By contrast, in vertebrates the clustered protocadherins (Pcdhs) provide analogous cell-surface diversity, but in this case generated through stochastic alternative promoter choice. Biophysical measurements with domain-deleted proteins showed that Pcdhs also interact in cis, through a membrane-proximal dimer interface involving extracellular cadherin domain 6 (EC6) and potentially EC5. The specificity-determining cell-cell recognition interface of Pcdhs involves domains EC1–4, as shown experimentally through mutagenesis analysis and suggested by mutation correlation analysis.

Crystallization screening of these dimeric γ-Pcdh fragments yielded crystals of γA1EC1–4, γA8EC1–4, γA9EC1–5, γB2EC1–5, and γB7EC1–4, and their structures were determined by molecular replacement. The γB2EC1–5 and γB7EC1–4trans dimer structures show the same overall arrangement as the previously published γB3EC1–4 trans dimer structure. For example, EC2:EC3 interacting residues 111 and 294 in the majority of γB2 orthologs (not including mouse) are lysine and aspartic acid, which are likely to form a salt bridge in the trans homodimer, whilst in γB3 and γB7 residue 111 is a conserved glutamic acid, which in the homodimeric complexes interacts favorably with H/R294 in γB3 or S294 in γB7. However hypothetical heterodimers between γB2 and γB3 or γB7 would juxtapose like charges E111 (γB3/7):D294 (γB2) and K111 (γB2):H/R294 (γB3) which would disfavor the heterophilic interactions (γB7 numbering). (E) Structural alignment of the overlapping EC3–5 regions of the γB2EC1–5 dimer with the γB2EC3–6 structure provides a model for the overall architecture of γB EC1–6 dimers.

>[2x]DQIRYSIPEELAKNSIVGNLARDLGLSVQNLPTRKLRVSAEKDYFTVNPESGDLLVGDRIDREQVCGKQPQCVLEFDIVAEKPLNIFHVAVILQDVNDNAPLFKQSEVDLNIGESTRPGKAFPLDPALDLDAGSNSLQKYYLTDNEYFEVTEKETPDGRKYPELILKRFLDREEHNFHQLVLTAVDGGDPPRSGTTQIRIQVTDINDNPPMFSQDVFSVTLREDVPPGFSVLQVTATDQDEGVNAEITYAFHNVDEQVERIFNLDKRTGEITTKDNLDFETAKSYTLNVEAKDPGDLASHCSIQVKILDENDCVPEVIVTSVFTPLPEDSPLGTVIALIKTRDRDSGENGDVYCHVLGNEGFVLKSSSKNYYKLVTDRTLDREAIPEYNVTIVAADRGKPPLSSNVIITLHISDVNDNAPVFHQASYLVHVAENNPPGTSIAQVSASDPDLGSNGLISYSIIASDLEPRALSSFVSVNQDSGVVFAQRAFDHEQLRSFQLTLQARDHGSPTLSANVSMRVLVGDRNDHHHHHHHH> MKINIIKAFGILLCRLKKYNPVTTGDINKFEFLFLKASYADKHWTPPKGLHENNESGLETAVRETLEETGINKDKYKLLNYQKTLKY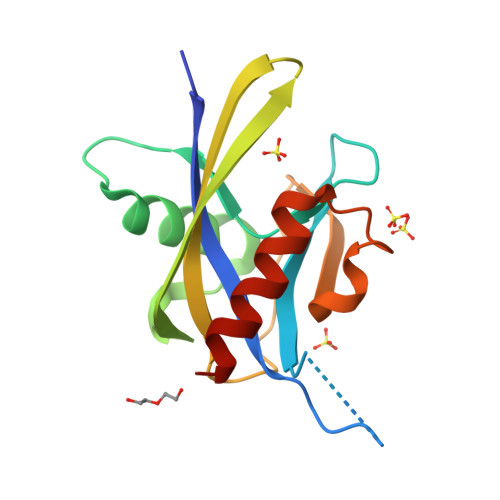NVKDKPKETTYYLAMLLNNEENVILSDEHTDYKWIGSHESDTYNLPESLADLLKEAEEFLNKEQL> XAYHGAPHEIRNRYQHDRALEILDRQYSRDSYIYAHLVLYMKDSSLQIIRAQNPRIISRSYNWDQLVLPNYRINDEKYYGRSELRHLRDGLLSDNGGRSQHDKGMNEPVSFQFIVQGDVDLGSVWFRVNKYNNISSSSFAMEAVSERAENYIGPLMRPIRYFDREM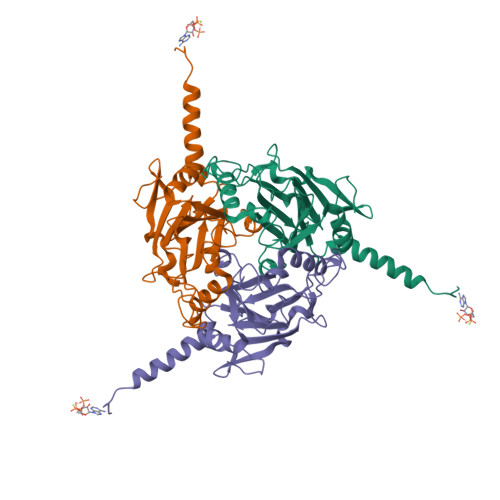AWSYVGKFDGILFPCHPVISFAVQRANRDGAGLYNGENIYKTLIRLNDSPDLYAHYDDEETSVANYWTRFQYLYRTKCDIAV2-amino-3-methyl-6-[(1S,2R)-2-phenylcyclopropyl]pyrimidin-4(3H)-one | C14 H15 N3 O 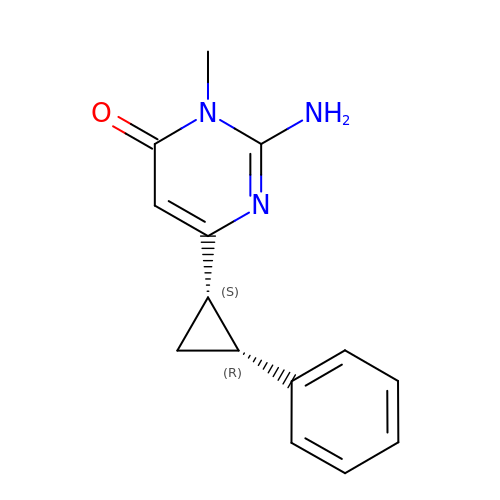| VTVXXFGROBMFAL-QWRGUYRKSA-N1-{7-cyclohexyl-6-[4-(4-methylpiperazin-1-yl)benzyl]-7H-pyrrolo[2,3-d]pyrimidin-2-yl}methanamine 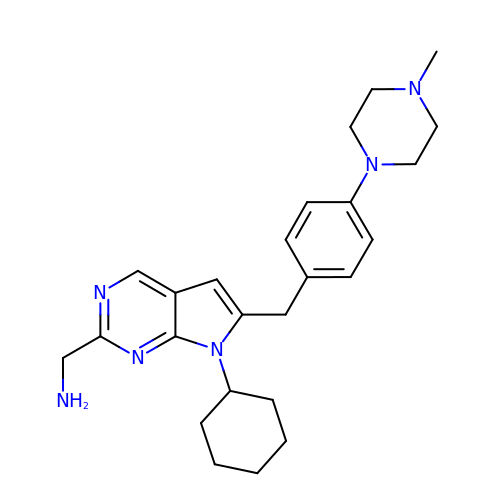| C25 H34 N6 | GCJSOJRPNOWSEH-UHFFFAOYSA-N> GAPVPVDENDEGLQRALQFAMAEYNRASNDKYSSRVV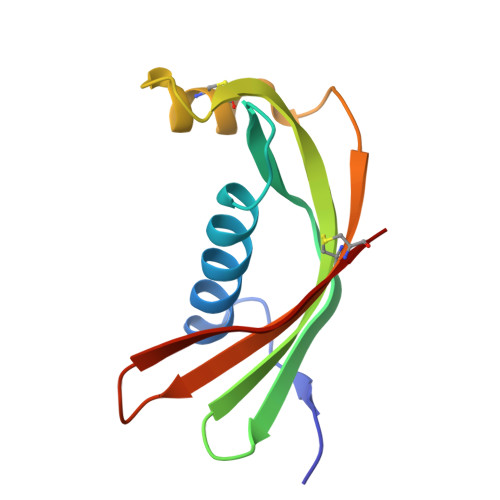RVISAKRQLVSGIKYILQVEIGRTTCPKSSGDLQSCEFHDEPEMAKYTTCTFVVYSIPWLNQIKLLESKCQ N~2~-[4-(4-phenylthiophen-2-yl)benzoyl]-L-alpha-glutamine | C22 H20 N2 O4 S | 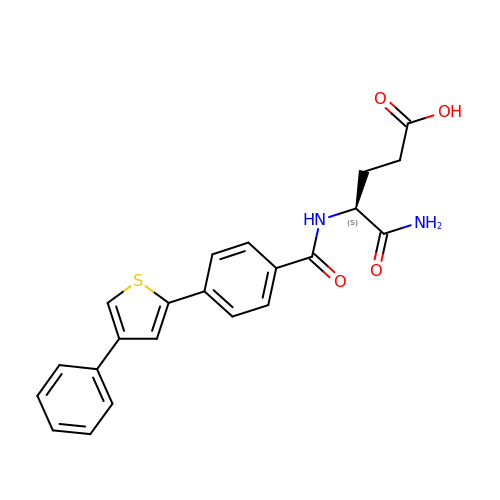ADDJDJQFPKUMAF-SFHVURJKSA-N> MSGTGITKPNSNSLPSGYRFNEFEIQEAIGEGGFGIVYRAYDHQLERTIAIKEYMPTSLAKRNDDLSIGLRGERFGKTFQA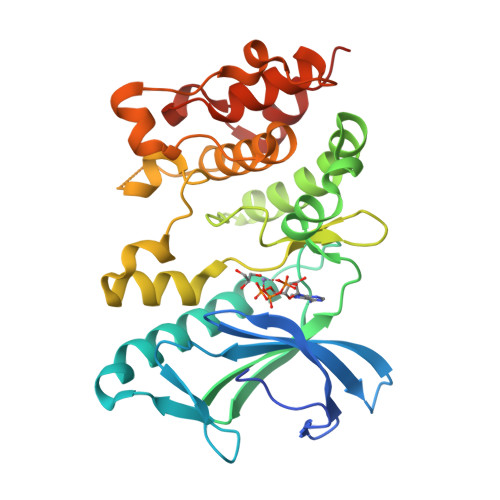GLNSFIQEARLLARFSHPGLLHVLRFWEENGTAYMGTQFYSGTTLKNLQAQQPEKIDEAWIRRLLPPLFSAINTIHQEGYLHRDISLDNIQIQESQLPVLLDFGSARKEIGNLSDETEIVLKPGFAPIEQYTENSDGEQGPWTDIYALGAVLHTLIVGSPPPVSVVRSIEDSYQPLTERRPAGYSPELLRTVDRALALKPEDRPQTIDEMAELLEHHHHHH>SNAAMLTFDALAETSEFARKWVPFVKKYNIEP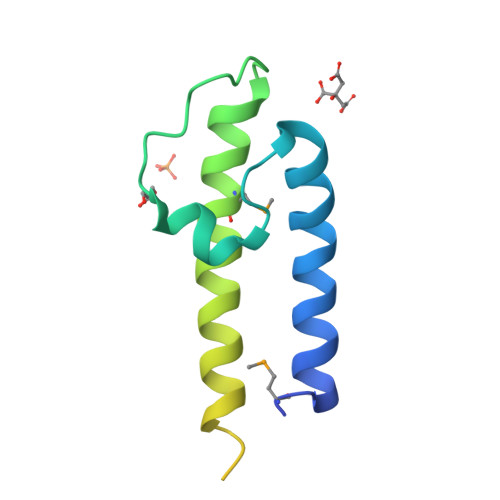RAPEWYFSQKIDYLKDKVHPSFVKDRRAMKREYEEFKVRINGLVAKAQKVPEEGWIMQDGTPWPGNNTRDHPGMIQVFLGHSGGLDTEGNELPRLV[2x]Phospholipid PG(16:0/cy17:0) | C39 H75 O10 P | 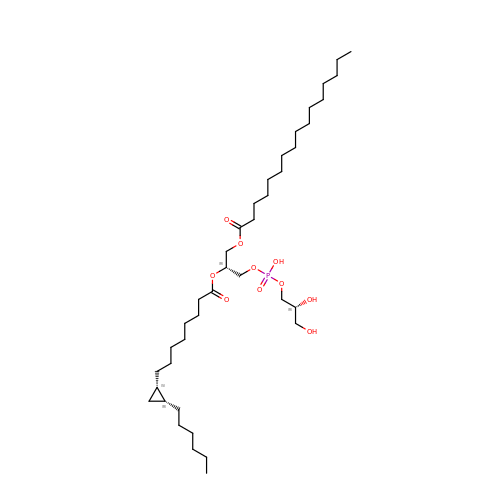JWIOKCJPLNKYBQ-UPIAJAFBSA-N> VATAAAVTAGVAIAKTIRLESEVTAIKNALKKTNEAVSTLGNGVRVLATAVRELKDFVSKNLTRAINKNKCDIADLKMAVSFSQFNRRFLNVVRQFSDNAGITPAI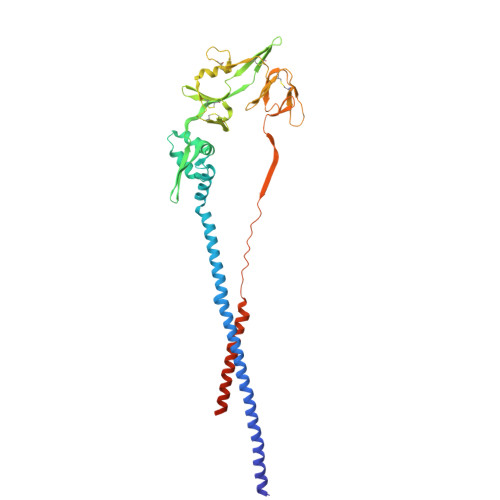SLDLMTDAELARAVSNMPTSAGQIKLMLENRAMVRRKGFGILIGVYGSSVIYMVQLPIFGVIDTPCWIVKAAPSCSEKKGNYACLLREDQGWYCQNAGSTVYYPNEKDCETRGDHVFCDTAAGINVAEQSKECNINISTTNYPCKVSTGRHPISMVALSPLGALVACYKGVSCSIGSNRVGIIKQLNKGCSYITNQDADTVTIDNTVYQLSKVEGEQHVIKGRPVSSSFDPVKFPEDQFNVALDQVFESIENSQALVDQSNRILSSAEKGNTSGRENLYFQ> MADTLESSLEDPLRSFVRVLEKRDGTVLRLQQYSSGGVGCVVWDAAIVLSKYLETPEFSGDGAHALSRRSVLELGSGTGAVGLMAATLGADVVVTDLEELQDLLKMNINMNKHLVTGSVQAKVLKWGEEIEGFPSPPDFILMADCIYYEE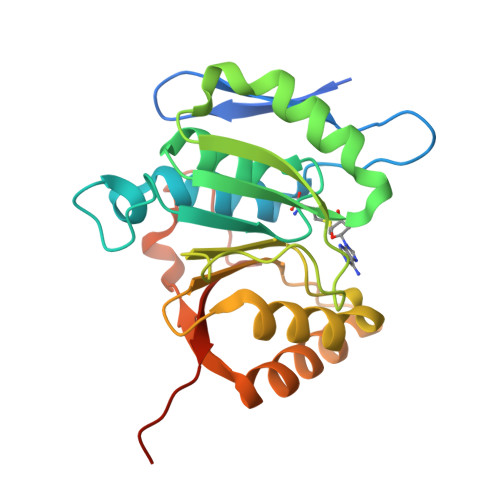SLEPLLKTLKDISGFETCIICCYEQRTMGKNPEIEKKYFELLQLDFDFEKIPLEKHDEEYRSEDIHIIYIRKKKSKFPSHHHHHH> KVAYLTFDDGPGKYTAELLNTLKQHDAKATFFLIGANVKEFPDLVKRENAEGHYVGMHSMTHNFAKLYKNGEYVNEMKEDQGLIANIIGKSPKLTRPPYGSMPGLNEGLRNKVVEGGFKVWDWTIDSLDWRY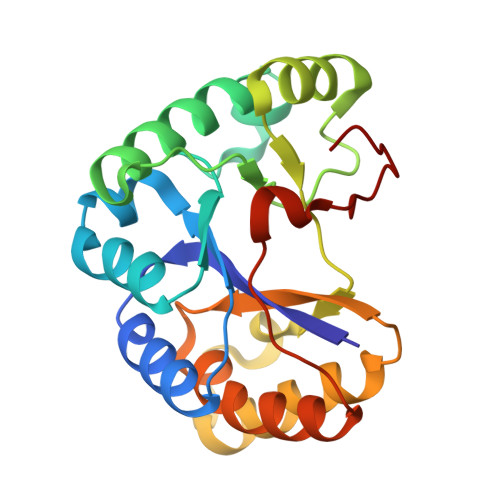NKMPVDAAAAQIAQNVLTNATKPQEVILMHDIHPQSVAAVPAILKGLKEKGYEFEAYHEESHFPVNFWHDNRM> GTA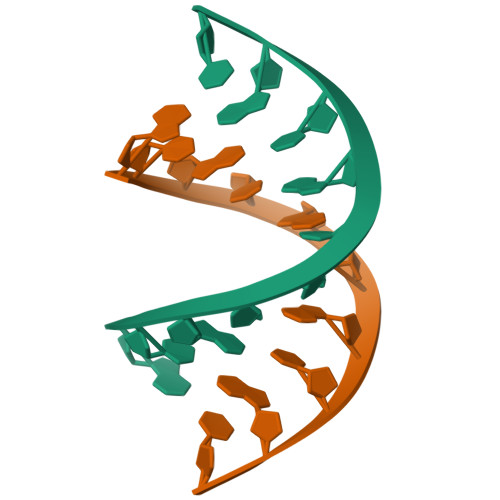CGCGTAC> NGDRLYRADSRPPDEIKRSGG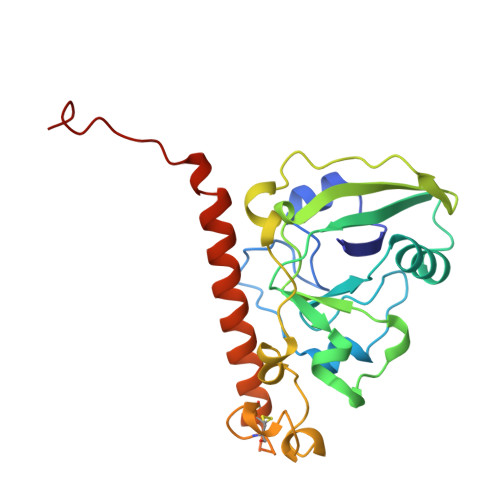LMPRGHNEYFDRGTQMNINLYDHARGTQTGFVRYDDGYVSTKLSLRSAHLAGQSILSGYSTYYIYVIATAPNMFNVNDVLGVYSPHPYEQEVSALGGIPYSQIYGWYRVNFGVIDERLHRNREYRDRYYRNLNIAPAEDGYRLAGFPPDHQAWREEPWIHHAPQGCGNSSNSSRTITRTITGDTCNEETQNLSTIYLREYQSKVKRQIFSDYQSEVDIYNRIRDEL> IVGGYTCGANTVPYQVSLNSGYHFCGGSLINSQWVVSAAHCYKSGIQVRLGEDNINVVEGNEQFISASKSIVHPSYNSETYNNDIMLIKLKSAASLNSRVASISL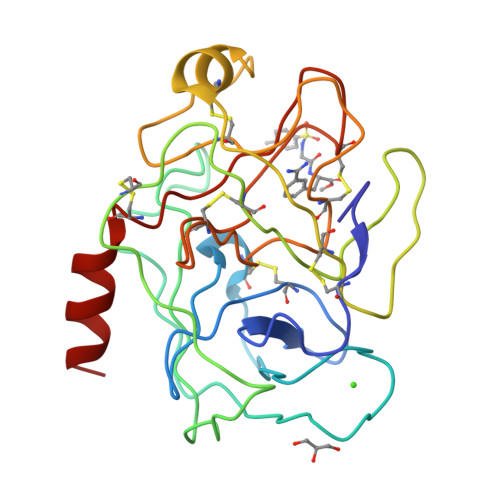PTSCASAGTQCLISGWGNTKSSGTSYPDVLKCLKAPILSDSSCKSASSFIITSNMFCVGYLEGGKDACQGDSGGPVVCSGKLQGIVSWGEGCAQKNKPGFYTKVCNYVSWIKQTIASN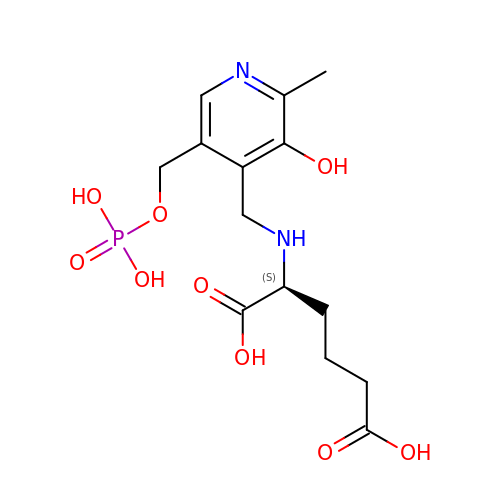(2S)-2-[({3-hydroxy-2-methyl-5-[(phosphonooxy)methyl]pyridin-4-yl}methyl)amino]hexanedioic acid | C14 H21 N2 O9 P | VAICOQQXLDOKQG-NSHDSACASA-N1.7.6 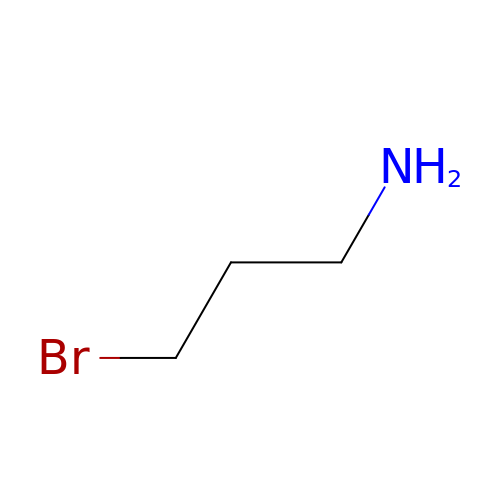3-bromanylpropan-1-amine  | C3 H8 Br N | ZTGQZSKPSJUEBU-UHFFFAOYSA-N>[4x]AMEFVNKQFNYKDPVNGVDIAYIKIPNAGQMQPVKAFKIHNKIWVIPERDTFTNPEEGDLNPPPEAKQVPVSYYDSTYLSTDNEKDNYLKGVTKLFERIYSTDLGRMLLTSIVRGIPFWGGSTIDTELKVIDTNCINVIQPDGSYRSEELNLVIIGPSADIIQFECKSFGHEVLNLTRNGYGSTQYIRFSPDFTFGFEESLEVDTNPLLGAGKFATDPAVTLAHELIHAGHRLYGIAINPNRVFKVNTNAYYEMSGLEVSFEELRTFGGHDAKFIDSLQENEFRLYYYNKFKDIASTLNKAKSIVGTTASLQYMKNVFKEKYLLSEDTSGKFSVDKLKFDKLYKMLTEIYTEDNFVKFFKVLNRKTYLNFDKAVFKINIVPKVNYTIYDGFNLRNTNLAANFNGQNTEINNMNFTKLKNFTGLFEFYKLLCVDEMEENLTQVGSILGNLKDMALNIGNEIDAQNRQIKRITDKADTNRDRIDIANARAKKLIDSANSALALQ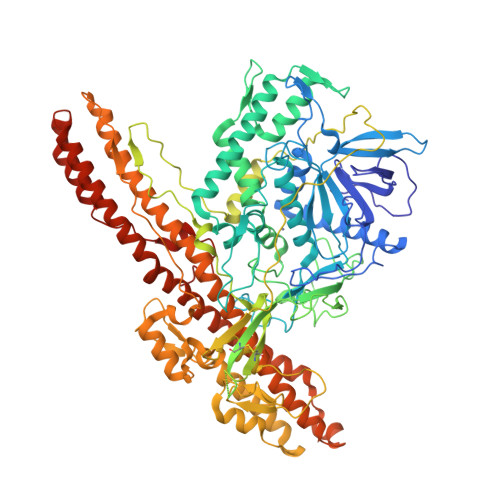CIKVNNWDLFFSPSEDNFTNDLNKGEEITSDTNIEAAEENISLDLIQQYYLTFNFDNEPENISIENLSSDIIGQLELMPNIERFPNGKKYELDKYTMFHYLRAQEFEHGKSRIALTNSVNEALLNPSRVYTFFSSDYVKKVNKATEAAMFLGWVEQLVYDFTDETSEVSTTDKIADITIIIPYIGPALNIGNMLYKDDFVGALIFSGAVILLEFIPEIAIPVLGTFALVSYIANKVLTVQTIDNALSKRNEKWDEVYKYIVTNWLAKVNTQIDLIRKKMKEALENQAEATKAIINYQYNQYTEEEKNNINFNIDDLSSKLNESINKAMININKFLNQCSVSYLMNSMIPYGVKRLEDFDASLKDALLKYIYDNRGTLIGQVDRLKDKVNNTLSTDIPFQLSKYVDNQRLLSTLEAHHHHHHHHHH>GSMAVTNVAELNALVERVKKAQREYASFTQEQVDKIFRAAALAAADARIPLAKMAVAESGMGIVEDKVIKNHFASEYIYNAYKDEKTCGVLSEDDTFGTITIAEPIGIICGIVPTTNPTSTAIFKSLISLKTRNAIIFSPHPRAKDATNKAADIVLQAAIAAGAPKDLIGWIDQPSVELSNALMHHPDINLILATGGPGMVKAAYSSGKPAIGVGAGNTPVVIDETADIKRAVASVLMSKTFDNGVICASEQSVVVVDSVYDAVRERFATHGGYLLQGKELKAVQDVILKNGALNAAIVGQPAYKIAELAGFSVPENTKILIGEVTVVDESEPFAHEKLSPTLAMYRAKDFEDAVEKAEKLVAMGGIGHTSCLYTDQDNQPARVSYFGQKMKTARILINTPASQGGIGDLYNFKLAPSLTLGCGSWGGNSISENVGPKHLINKKTVAKRAENMLWHKLPKSIYFRRGSLPIALDEVITDGHKRALIVTDRFLFNNGYADQITSVLKAAGVETEVFFEVEADPTLSIVRKGAELANSFKPDVIIALGGGSPMDAAKIMWVMYEHPETHFEELALRFMDIRKRIYKFPKMGVKAKMIAVTTTSGTGSEVTPFAVVTDDATGQKYPLADYALTPDMAIVDANLVMDMPKSLCAFGGLDAVTHAMEAYVSVLASEFSDGQALQALKLLKEYLPASYHEGSKNPVARERVHSAATIAGIAFANAFLGVCHSMAHKLGSQFHIPHGLANALLICNVIRYNANDNPTKQTAFSQY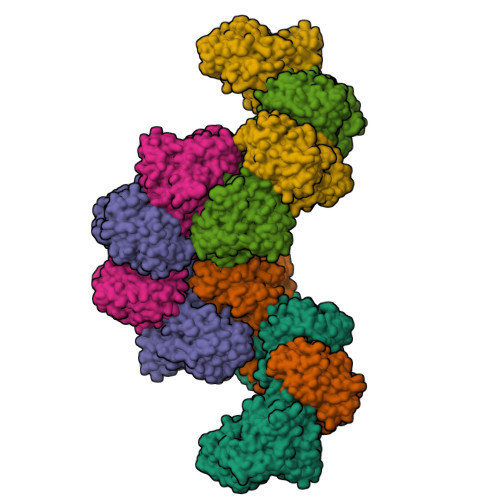DRPQARRRYAEIADHLGLSAPGDRTAAKIEKLLAWLETLKAELGIPKSIREAGVQEADFLANVDKLSEDAFDDQCTGANPRYPLISELKQILLDTYYGRDYVEGETAAKKEAAPAKAEKKAKKSA[6x]> APLKLYGMPLSP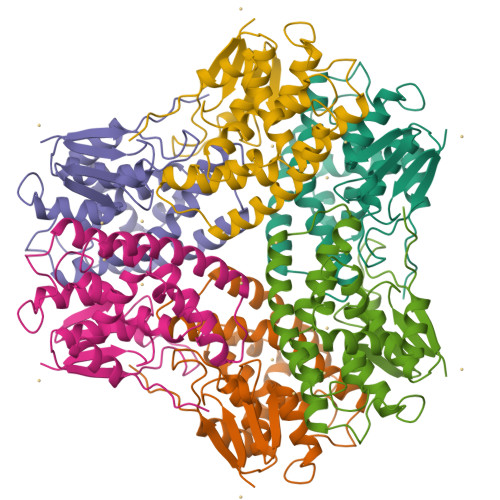NVVRVATVLNEKGLDFEIVPVDLTTGAHKQPDFLALNPFGQIPALVDGDEVLFESRAINRYIASKYASEGTDLLPATASAAKLEVWLEVESHHFYPNASPLVFQLLVRPLLGGAPDAAVVDKHAEQLAKVLDVYEAHLARNKYLAGDEFTLADANHASYLLYLSKTPKAGLVAARPHVKAWWEAIVARPAFQKTVAAIPLPPPP>[2x]GAMTLPAEGEIGLIDVGSLQLESGAVIDDVCIAVQRWGKLSPARDNVVVVLHALTGDSHITGPAGPGHPTPGWWDGVAGPGAPIDTTRWCAVAT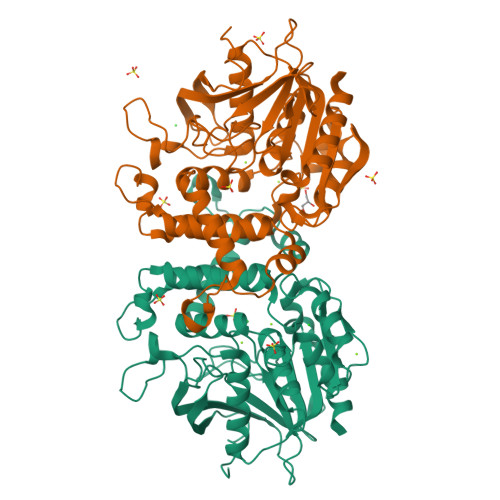NVLGGCRGSTGPSSLARDGKPWGSRFPLISIRDQVQADVAALAALGITEVAAVVGGSMGGARALEWVVGYPDRVRAGLLLAVGARATADQIGTQTTQIAAIKADPDWQSGDYHETGRAPDAGLRLARRFAHLTYRGEIELDTRFANHNQGNEDPTAGGRYAVQSYLEHQGDKLLSRFDAGSYVILTEALNSHDVGRGRGGVSAALRACPVPVVVGGITSDRLYPLRLQQELADLLPGCAGLRVVESVYGHDGFLVETEAVGELIRQTLGLAD>[2x]MSQEELRQQIAELVAQYAETAMAPKPFEAGKSVVPPSGKVIGTKELQLMVEASLDGWLTTGRFNDAFEKKLGEYLGVPYVLTTTSGSSANLLALTALTSPKLGVRALKPGDEVITVAAGFPTTVNPTIQNGLIPVFVDVDIPTYNVNASLIEAAVSDKTKAIMIAHTLGNL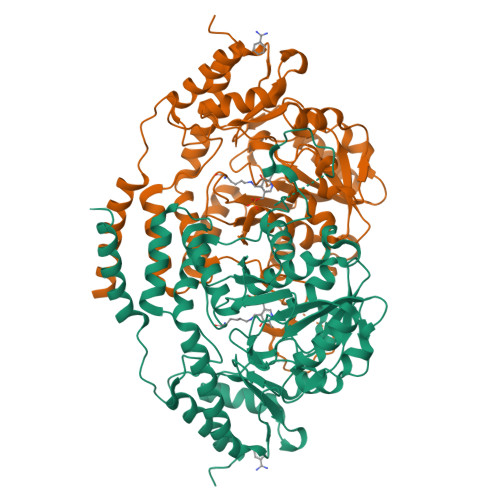FDLAEVRRVADKYNLWLIEDCCDALGSTYDGKMAGTFGDIGTVSFYPAKHITMGEGGAVFTQSAELKSIIESFRDWGRDCYCAPGCDNTCKKRFGQQLGSLPFGYDHKYTYSHLGYNLKITDMQAACGLAQLERIEEFVEKRKANFKYLKDALQSCADFIELPEATENSDPSWFGFPITLKEDSGVSRIDLVKFLDEAKVGTRLLFAGNLTRQPYFHDVKYRVVGELTNTDRIMNQTFWIGIYPGLTHDHLDYVVSKFEEFFGLNF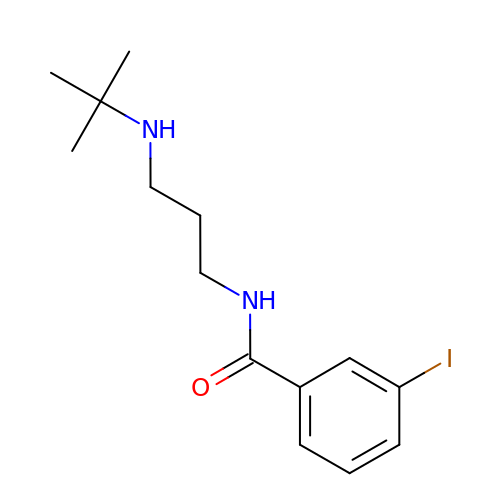N-[3-(tert-butylamino)propyl]-3-iodobenzamide | C14 H21 I N2 O | YKQSWTFGSUNNEI-UHFFFAOYSA-N>[2x]SNADAESLFREALSNKVDELAHFLLRKYRAKELVTKAEMLERVIKNYKRCFPVIFGKASESLKMIFGIDVKEVDPTSNTYTLVTCLGLSYDGLLGNNQIFPKTGLLIIVLGTIAMEGDSASEEEIW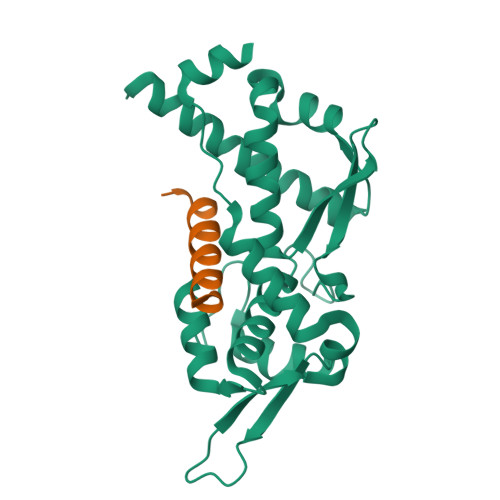EELGVMGVYDGREHTVYGEPRKLLTQDWVQENYLEYRQVPGSNPARYEFLWGPRALAETSYVKVLEHVVRVNARVRIAYPSLREAALLEEEEGV;>[2x]HSKYRKKHKSEFQLLVDQARKGYKKIAG> MSSSIDISKINSWNKEFQSDLTHQLATTVLKNYNADDALLNKTRLQKQDNRVFNTVVSTDSTPVTNQKSSGRCWLFAATNQLRLNVLSELNLKEFELSQAYLFFYDKLEKANYF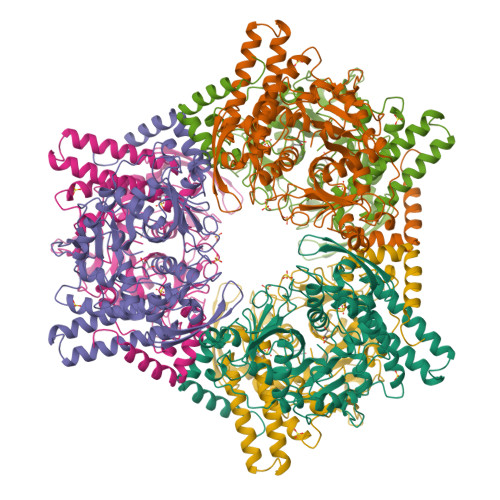LDQIVSSADQDIDSRLVQYLLAAPTEDGGQYSMFLNLVKKYGLIPKDLYGDLPYSTTASRKWNSLLTTKLREFAETLRTALKERSADDSIIVTLREQMQREIFRLMSLFMDIPPVQPNEQFTWEYVDKDKKIHTIKSTPLEFASKYAKLDPSTPVSLINDPRHPYGKLIKIDRLGNVLGGDAVIYLNVDNETLSKLVVKRLQNNKAVFFGSHTPKFMDKKTGVMDIELWNYPAIGYNLPQQKASRIRYHESLMTHAMLITGCHVDETSKLPLRYRVENSWGKDSGKDGLYVMTQKYFEEYCFQIVVDINELPKELASKFTSGKEEPIVLPIWDPMGALAK> K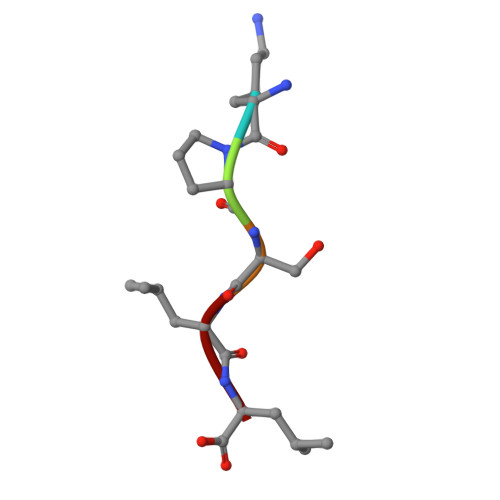PSLL>KPFTLPILTLGELTNSRFPLPIDVLYTNPNESAIVQCQNGRCTLDGELQGTTQLLPTGICAFRGKVTQQVQDEHRGTHWNMTVTNLNGTPFDPTEDVPAPLGTPDFSGQIYGVISQRNTNTVPGEGNLPANRAHEAVIATYSPKFTPKLGNIQFSTWETQDVSSGQPTKFTPVGLASVDANSHFDQWTLPSYSGALTLNMNLAPSVAPVFPGECLLFFRSFIPLKGGYGNPAIDCLMPQEWVQHLYQESAPSLSDVALVRYVNPETGRTLFEAKLHRNGFLTVARNSAGPVVAPTNGYF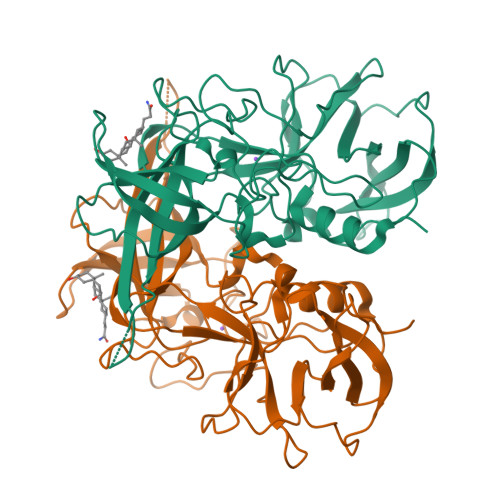RFDSWVNQFYTLAPM[2x]>[2x]MLRIIDTET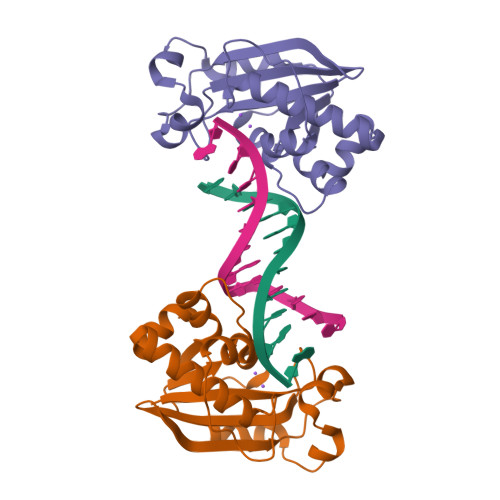CGLQGGIVEIASVDVIDGKIVNPMSHLVRPDRPISPQAMAIHRITEAMVADKPWIEDVIPHYYGSEWYVAHNASFDRRVLPEMPGEWICTMKLARRLWPGIKYSNMALYKTRKLNVQTPPGLHHHRALYDCYITAALLIDIMNTSGWTAEQMADITGRLEHHHHHH> MALSIKHPEADRLARALAARTGETLTEAVVTALRERLARETGRARVVPLRDELAAIRHRCAALPV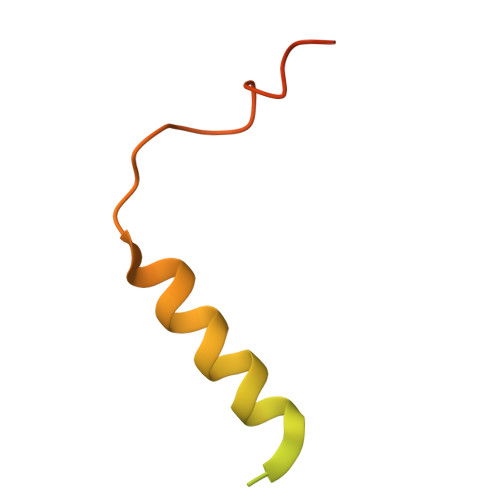VDNRSAEAILGYDERGLPA>[7x]MWADIYHKLVEIYDIKAVKFLLDVLKILIIAFIGIKFADFLIYRFYKLYSKSKIQLPQRKIDTLTSLTKNAVRYIIYFLAGASILKLFNIDMTSLLAVAGIGSLAIGFGAQNLVKDMISGFFIIFEDQFSVGDYVTINGISGTVEEIGLRVTKIRGFSDGLHIIPNGEIKMVTNLTKDSMMAVVNIAFPIDEDVDKIIEGLQEICEEVKKSRDDLIEGPTVLGITDMQDSKLVIMVYAKTQPMQKWAVE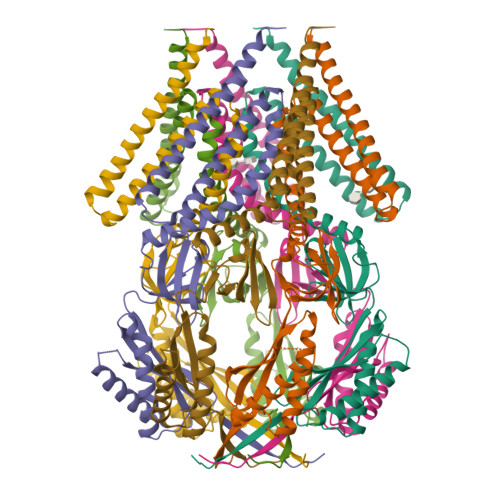RDIRYRVKKMFDQKNISFPYPRTTVILSEKKTN> AE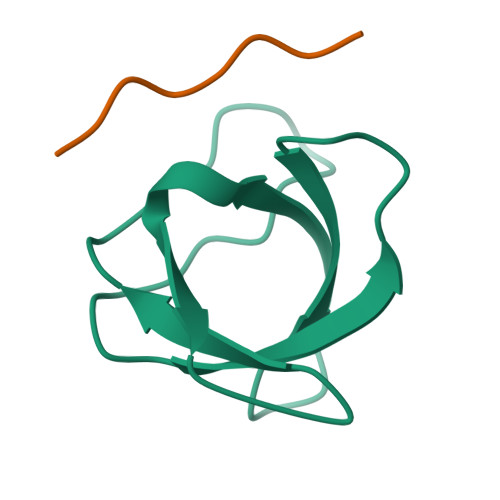YVRALFDFNGNDEEDLPFKKGDILRIRDKPEEQWWNAEDSEGKRGMIPVPYVEKY;> PPPVPPRRRR> QDNSRYTHFLTQHYDAKPQGRDDRYCES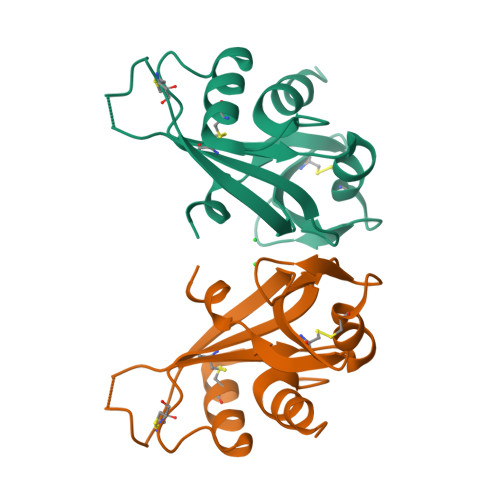IMRRRGLTSPCKDINTFIHGNKRSIKAICENKNGNPHRENLRISKSSFQVTTCKLHGGSPWPPCQYRATAGFRNVVVACENGLPVHLDQSIFHRP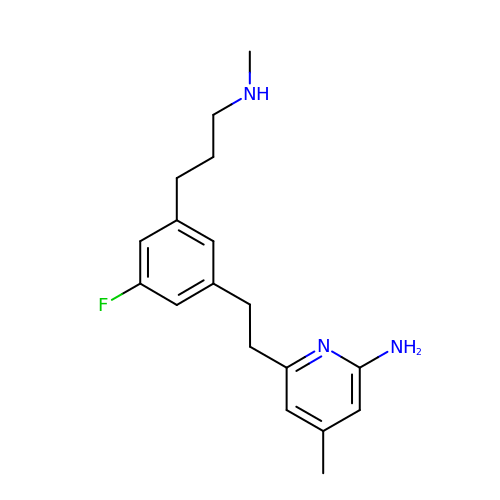6-(2-{3-fluoro-5-[3-(methylamino)propyl]phenyl}ethyl)-4-methylpyridin-2-amine | C18 H24 F N3 | PEJWJTGGAYICCM-UHFFFAOYSA-N> MAHHHHHHSAALEVLFQGPGQPGFCIKTNSSEGKVFINICHSPSIPPPADVTEEE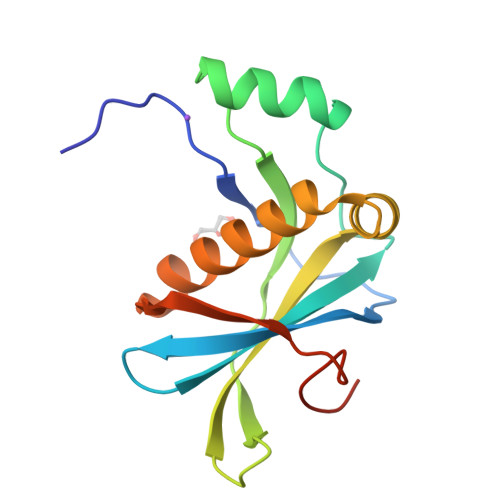LLQMLEEDQAGFRIPMSLGEPHAELDAKGQGCTAYDVAVNSDFYRRMQNSDFLRLLVIRIARQGLEYKYDLRLAPPWDMMKNRPFMGSISQQNIR> MFFRFHSTTLQTCLTSGVARSSVAVAVPLRAGCTRREMSSGGDGVLEGAMHKPGESGLQAGSSTTIAGKETWSQFSTKMRYGRRRIRVIDVAAKMSYEYQMLRKMCKRRPAMRQWAVRDDFCDMNPGVVIMSPSMQAAFMKVFRMKEKGLIRQCLRDIVPVIEYRNREEPARLPTNPADMIPEGEPDTLNQKKRELFERREKGENFADLRLHDKRSQAKLRFRIRQRLLKFQRQLAVANAIASRSVL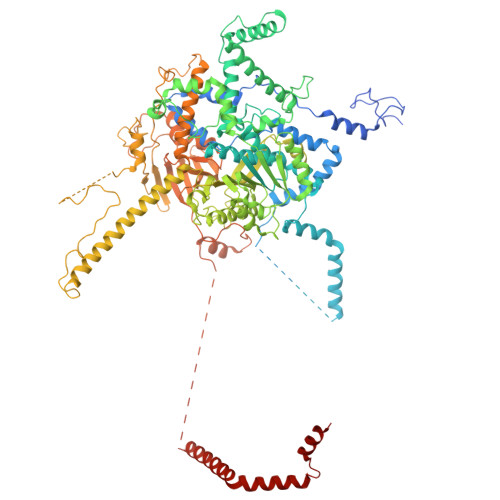YSTNDAIGYFLFRGAAMYAGMHRVFFELSKQLPHFVPKTMLDFGAGTGTAILVAKEVYDPGSLAYPLYRSLRQTMQGNDSSRTHQLSELRYDLKRLQRNNEEKKKVRFMAVAALLERGEVDPADLPEDLKREIAEVATAAATAKKDRLVREAHARYRDVVDGTEWESGDPLGEVRASTEDPEDVIDGEQGDGGDDGEAAKGRPKTWWEKLIDVENETARTRAARRLRPLQEVTAVEPSPGMMEIGTMVLHDDVPNVTWKRYLLPEDEAIQHDLVVAAYSLSEIATSENRRRIVQQLWKMTKGVLVFVEFANLNNFNILMEARDWILEEKDVGLWDWQPTIVAPCPHEHRCPLRHCKTGVKRKRMRICSTEAHYRSTFVEVWARHMPLKVGIEPISYLILARNELVPERAERRREQLKKAEEMKRRERDVKQQQLHEASLAVKDVVFERLSDEALHRVQSSVPQPLTDIDEVREASTSATSTSLLKDLKDGATSTGEIGHMPTDVPRLVKTGNTRHNRLIFPLQFPPATHKFNRAFVDAGYQRQRAITPAEMLVVRQEVEQLQQRVMRAAPKYLRVVRDPRCHGKVQADFCTPEGDLVSGRVYRRFYGDRNRVSAHSTMRWQHIGGWKLLKRIRRGSLFPHNVPLYAVTKHAQIDFPNTLLDTKHSTVEQTAMQYNDPMSLVEMPDDGLTREELKQKRRLQRDVELQKKVEEKLEDIFGVNAKDWKTDDLGGGRLDARREISEQQWADAVRRAKIRTVQHTKNALPFAAKKRAAQRALQVRRRNVRLEMSGNRRR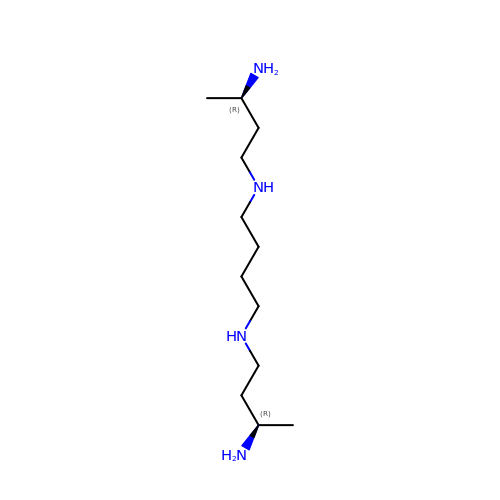(3R,3'R)-N~1~,N~1~'-butane-1,4-diyldibutane-1,3-diamine | C12 H30 N4 | LXKFTCVCBKNJNM-VXGBXAGGSA-N> PMYEVQWKVVEEINGNNYVYIDPTQLPYDHKWEFPRNRLSFGKTLGAGAFGKVVEATAYGLIKSDAAMTVAVKMLKPSAHLTEREALMSELKVLSYLGNHMNI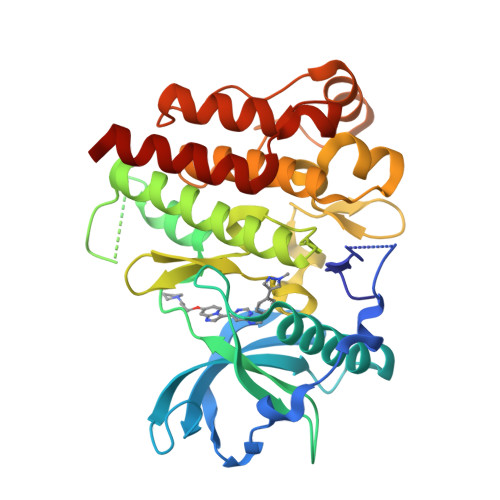VNLLGACTIGGPTLVITEYCCYGDLLNFLRRKRDSFICSKTEPAIMEDDELALDLEDLLSFSYQVAKGMAFLASKNCIHRDLAARNILLTHGRITKICDFGLARDIKNDSNYVVKGNARLPVKWMAPESIFNCVYTFESDVWSYGIFLWELFSLGSSPYPGMPVDSKFYKMIKEGFRMLSPEHAPAEMYDIMKTCWDADPLKRPTFKQIVQLIEKQISESTNHI The operon spr0693-spr0694-spr0695 of S. pneumoniae R6 encodes a putative ABC transporter that contributes to the resistance of antibiotics and antimicrobial peptides. Sequence analyses suggest that the Spr0693–0694–0695 assembly is similar to Escherichia coli MacAB, with Spr0693 and Spr0694–0695 corresponding to MacA and MacB, respectively. Here we present the crystal structures of S. pneumoniae Spr0694–0695 and Spr0693, representing the structure of a MacAB-like efflux pump in Gram-positive bacteria. In summary, the structure of Spr0694-Spr0695 reveals some features for this family of ABC transporters, which are characterized by a unique 8-TM fold and an ECD/PLD insertion between TM1 and TM2.

As initial efforts to get the full-length structure of Spr0693 failed after exhaustive trials, we made a series of truncations and finally a truncated version (Ser59–Lys324) without the membrane-proximal (MP) domain, enabled us to solve the structure at 3.0 Å. The quaternary structure of Spr0693 displays a typical hexameric nanotube, similar to the previously reported MFP structures. The two outermost α-helices form a twisted left-handed α-helical hairpin domain; and six helical hairpins further pack into a cylindrical assembly to form an α-helical barrel of 31 Å in diameter and 56 Å in height. The 24-Å high lipoyl domain at the middle harbors two layers of three-stranded β-sheets packing against each other, with a topology similar to the biotinyl/lipoyl carrier proteins and domain family. The β-barrel domain at the bottom is composed of six twisted anti-parallel β-strands and a short α-helix, which form a stacked β-barrel of 24 Å in height. The six lipoyl domains, as well as the six β-barrel domains, are aligned in a head-to-tail manner to form a double-layered ring-like structure in the quaternary structure. A top view of the Spr0693 cylinder structure reveals a narrow pore, which is formed by the loops (residues Asn211–Val224) from the lipoyl domains. These loops adopt a so-called turn-back conformation and point towards the center, forming a hexameric ring with the residue Gly220 at the innermost site. However, the glycine residue Gly220, as well as the loop, has a relatively higher B-factor, and the primary sequence of the loop is variable in the homologs of Spr0693, suggesting that the ring is structurally flexible and might have a rather broad spectrum of substrate selectivity. Structural superposition reveals that the hexameric Spr0693 shares an overall architecture quite similar to that of MacA, with an RMSD of 2.85 Å over 1226 Cα atoms.

>MSVLLSGTVTAKNEQYVYFDASKGDLDEILVSVGDKVSEGQALVKYSSSEAQAAYDSASRAVARADRHINELNQARNEAASAPAPQLPAPVGGEDATVQSPTPVAGNSVASIDAQLGDARDARADAAAQLSKAQSQLDAMTVLSTLEGTVVEVNSNVSKSPTGASQVMVHIVSNENLQVKGELSEYNLANLSVGQEVSFTSKVYPDKKWTGKLSYISDYPKNNGEAASPAAGNNTGSKYPYTIDVTGEVGDLKQGFSVNMEVKSKTKHHHHHH[3x]> GHMSRHDVTNATLETTGKELTETYMEMLNGDVVEVSIANEERIVSLLSSLASANVTLKQLIGTKIGVAVGQFLSDGFPPHIVRFSKGILDYWFRQLPEEVQKQL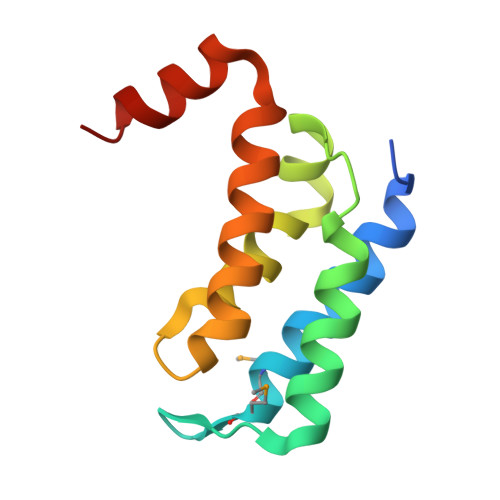LAKRALG>MIYMLGTNICVYAINKHPDSYYNNLELLAKNNTIAISSIVLAELQYGVSKSKKKEQNQSKLDIFLSRLEIIDFSAKCTFYYGELRTELEQKGLIIGNNDLLIASHAIAENATLVTNNIKEFKRIPNLILENWDK[4x];>MNKAKIFMNGQSQAVRLPKEFRFSVKEVSVIPLGKG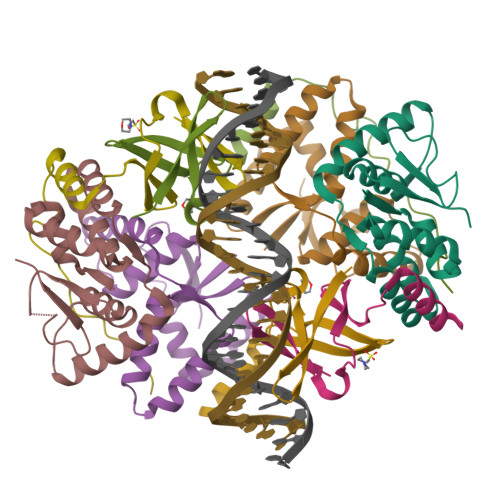IVLQPLPNSWKDVFQEMAEISSDDIFPEGRKDLPPQKRKYFE[4x]>MRIVAADTGGAVLDESFQPVGLIATVAVLVEKPYKTSKRFLVKYADPYNYDLSGRQAIRDEIELAIELAREVSPDVIHLNSTLGGIEVRKLDESTIDALQISDRGKEIWKELSKDLQPLAKKFWEETGIEIIAIGKSSVPVRIAE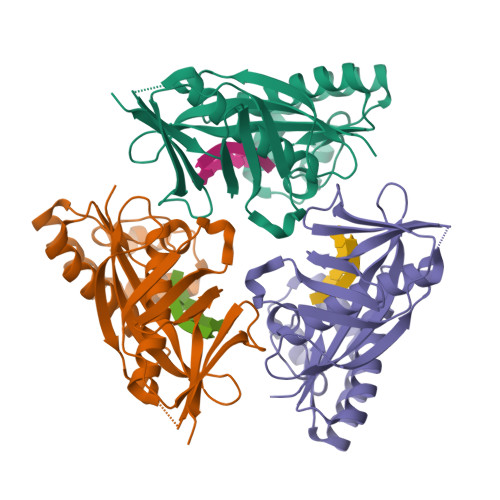IYAGIFSVKWALDNVKEKGGLLVGLPRYMEVEIKKDKIIGKSLDPREGGLYGEVKTEVPQGIKWELYPNPLVRRFMVFEITSKSHHHH[3x]>MGSITENTSWNKEFSAEAVNGVFVLCKSSSKSCATNDLARASKEYLPASTFKIPNAIIGLETGVIKNEHQVFKWDGKPRAMKQWERDLTLRGAIQVSAVPVFQQIAREVGEVRMQKYLKKFSYGNQNISGGIDKFWLEGQLRISAVNQVEFLESLYLNKLSASKENQL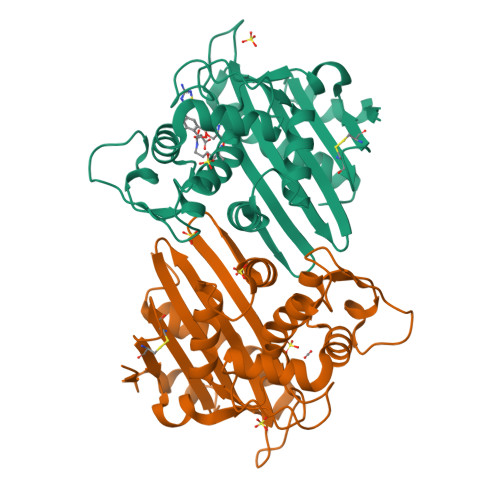IVKEALVTEAAPEYLVHSKTGFSGVGTESNPGVAWWVGWVEKETEVYFFAFNMDIDNESKLPLRKSIPTKIMESEGIIGG[4x]Lactobacillus casei produces a GH29A α-fucosidase, AlfC, that is ~104-fold more active on α(1-6)-fucosyl linkages compared to other linkages. This enzyme is particularly relevant because α(1-6) linkages form the basis of human core fucosylation, which significantly impacts the function of glycoproteins such as antibodies. AlfC is a single-domain enzyme that adopts a (β/α)8 fold typical of GH29 enzymes, with an active site at the center of the barrel. Our results suggest that AlfC employs a conserved hydrolytic mechanism with a specific subsite that accommodates GlcNAc in α(1,6)-linkages, while AlfC tranfucosidase mutants work by shifting equilibrium between open and closed conformations of an active-site loop.

In order to understand the α(1,6) specificity of AlfC, we solved the crystal structure of AlfCD200A bound to its preferred substrate, Fucα(1,6)GlcNAc. With fucose in the active site, GlcNAc sits in an aromatic subsite adjacent to the active site, formed by residues Y37, W40, and W158. This binding mode furthermore allows oxygen of the N-acetyl group to hydrogen bond with the backbone nitrogen of A154. N-linkages of this disaccharide (as seen on EndoS-treated IgG) can be readily accommodated, as C1 of GlcNAc (which connects to Asn297 of IgG) points away from the surface of the enzyme. In contrast, AlfC cannot accommodate longer carbohydrate linkages (as seen in untreated IgG), because O4 of GlcNAc (which connects to another GlcNAc) would point directly toward the surface of the enzyme, creating steric clashes for any polysaccharide longer than two residues. When the Fucα(1,6)GlcNAc crystal structure is superimposed over the closed state conformation from the molecular dynamics simulation, it is apparent that the closed state still accommodates the glycan well, with D200 and D242 flanking the reactive C1 of fucose. Our results provide the structural basis for α(1,6)-specificity of AlfC, identifying an aromatic +1 subsite adjacent to the active site that specifically accommodates GlcNAc in α(1,6)-linkages. They also provide a rationale for the requirement of endoglycosidase pre-treatment of antibodies before defucosylation, as additional sugars attached to the +1 sugar would clash with the enzyme surface.

>[4x]MNDNVAWFKQAKYGMMIHWGLYSLLAGEYRGESSSAYAEWIQSKFQIPNAEYGNLATAFNPLYFDAKKIVALAKQCGMQYLVVTTKHHDGFAMYHSKVDAYNVYDATPFHRDIIGELAEACQKAGLKFGLYYSQDLDWHDPNGGGYKSNDVETAGTTWDNSWDFPDEDQKNFDLCFDNKILPQIKEIMSNYGDIATAWFAVPMTLSEAQSQTIYDTVRELQPNCLINSRLGNGKYDFVSLGDNEIPKNKEDMNKTDVDYNEITGFKPSPLGLYETAGTINDSWGFSYHDQNWKTPRTLYRYKQHLNDFGINYLLNVGLDPLGRVPMMAEENLLAAKALEDEANRL>[6x]KEIVFGTTVGDFGDMVKEQIQPELEKKGYTVKLVEFTDYVRPN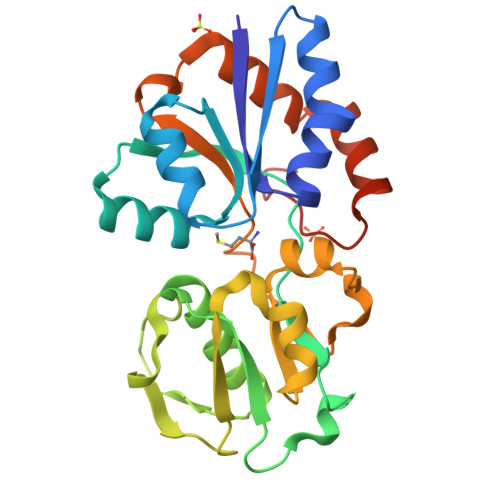LALAEGELDINVFQHKPYLDDFKKEHNLDITEVFQVPTAPLGLYPGKLKSLEEVKDGSTVSAPNDPSNFARVLVMLDELGWIKLKDGINPLTASKADIAENLKNIKIVELEAAQLPRSRADVDFAVVNGNYAISSGMKLTEALFQEPSFAYVNWSAVKTADKDSQWLKDVTEAYNSDAFKAYAHKRFEGYKSPAAWNEGAAK> ALEEAPWPPPEGAFVGFVLSRKEPMWADLLALAAARGGRVHRAPEPYKALRDLKEARGLLAKDLSVLALREGLGLPPGDDPMLLAYLLDPSNTTPEGVARRYGGEWTEEAGERAALSERLFANLWGRLEGEERLLWLYREVERPLSAVLAHMEATGVRLDVAYLRALSLEVAEEIARLEAEVFRLAGHPFNLNSRDQLERVLFDELGLPAIGKTEKTGKRSTSAAVLEALREAHPIVEKILQYRELTKLKSTYIDPLPDLIHPRTGRLHTRFNQTATATGRLSSSDPNLQNIPVRTPLGQRIRRAFIAEEGWLLVALDYSQIELRVLAHLSGDENLIRVFQEGRDIHTETASWMFGVPREAVDPLMRRAAKTINFGVLYGMSAHRLSQELAIPYEEAQAFIERYFQS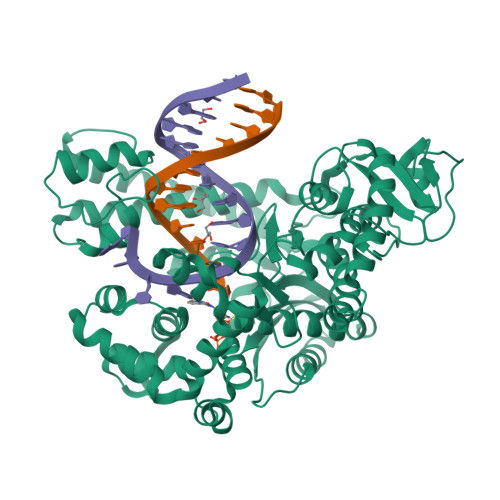FPKVRAWIEKTLEEGRRRGYVETLFGRRRYVPDLEARVKSVREAAERMAFNMPVQGTAADLMKLAMVKLFPRLEEMGARMLLQVHDELVLEAPKERAEAVARLAKEVMEGVYPLAVPLEVEVGIGEDWLSAKE> MRGSHHHHHHGIAGDTLGLTRPNESDAPKISIGAKDTAVVQWQGDLLAIGATENDMARDENSKFKNPLLQQLDSELNGLLSAASSEEDFSGKSGQSVNLRFPGGRITLVGLGSSASSPTSYHSLGQAAAAAAKSSQARNIAVALASTDGLSAESKINSASAIATGVVLGSFEDNRFRSESKKSTLESLDILGLGTGPEIERKIKYAEHVCAGVILGRELVNAPANIVTPAVLAEEAKKIASTYSDVISVNILDAEQCKELKMGAYLAVAAAATENPPYFIHLCFKTPTKERKTKLALVGKG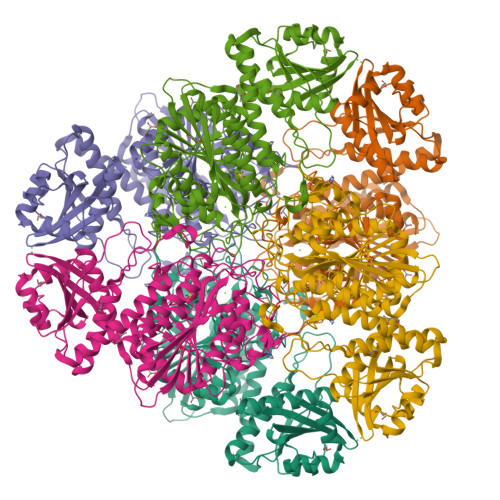LTFDSGGYNLKVGARSRIELMKNDMGGAAAVLGAAKALGEIRPSRVEVHFIVAACENMISAEGMRPGDIVTASNGKTIEVNNTDAEGRLTLADALIYACNQGVEKIIDLATLTGAIMVALGPSVAGAFTPNDDLAREVVEAAEASGEKLWRMPMEESYWESMKSGVADMINTGPGNGGAITGALFLKQFVDEKVQWLHLDVAGPVWSDEKKNATGYGVSTLVEWVLRN>MPFPEKFFWGASSSGFQFEMGDPEGKSIDPNTDWFKWVHDETNIRRGVVSGDLPEHGINYWDLFRSDHELAASIGMNAYRIGIEWSRIFPKPTLDVRVGIELDPEGYITRVEVDDKAIEELDLLANKEAVSRYREIILDLRDRGLKVFVCLNHFTLPLWIHDPIACRDTKLKRGPKGWVDKTTILEFAKYSAYMAWSLGNIVDYWVTFNEPMVVTEAGYFQPEVGFPPGLRNISAFKTACLNIANAHVVAYDLIKKYDKVRADDDSPSAAYVGIVHNIVPIKPYSERKLDLKAADLMNYIHNKWILEFIVRGKIDRSLVGREKYLIDKFKDKLDWLGVNYYTRIVLKGKWVPPLISPVPVIPDIVKGYGFNCTPGGRSLDGMPVSDFGWEVYPQGLSDALDIASEYGKPLIVTENGIADSEDNIRPYFLVSHLKVLEEYVEKKKNVYGYLHWALTDNYEWAQGFKMRFGLTDVDLETKERKPRESSEVFKIIASEKTVPEELVEKYPKPIF[2x]

Beta-glucosidase is an enzyme that catalyzes the hydrolysis of the glycosidic bonds of cellobiose, resulting in the production of glucose, which is an important step for the effective utilization of cellulose. In the present study, a thermostable β-glucosidase was isolated and purified from the Thermoprotei Thermofilum sp. ex4484_79 and subjected to enzymatic and structural characterization. A similarity search was performed with the BLAST program; the TsBGL protein was found to be a member the GH1 family. Members of the GH1 family have a (β/α)8-barrel domain structure that contains the active site, and the hydrolysis of the β-glycosidic bond is carried out via a catalytic mechanism that involves the action of two conserved glutamate residues that act as nucleophiles and proton donors.

The TsBGL crystal belonged to the space group P1211 and diffracted to a resolution of 2.14Å. The asymmetric unit of the crystal structure consisted of two protein molecules. The overall view indicates that TsBGL has a classic (β/α)8-barrel domain structure. The central (β/α)8 barrels consisted of eight parallel β-strands, namely β1 (Phe8-Ser13), β2 (Asn77-Ile83), β3 (Lys146-Asn152), β4 (Asp203-Asn209), β5 (Tyr271-Ile278), β6 (Trp335-Tyr340), β7 (Pro409-Glu414), and β8 (Asn445-His451), surrounded by eight α-helices, namely, α1 (Asn59-Ile74), α2 (Asn126-Arg143), α3 (Lys181-Gly199), α4 (Asn232-Asp258), α5 (Arg287-Asn302), α6 (Pro393-Glu405), α7 (Ile424-Lys444), and α8 (Arg483-Lys496). In TsBGL, Glu210 and Glu414 served as the putative catalytic residues. Glu414 was located at the end of β-strand 7, Glu210 was located behind Asn209, which was the end of β-strand 4, Glu210 is a proton donor, Glu414 is a catalytic nucleophile, and the closest distance between Glu210 and Glu414 was 4.5Å, which matched the catalytic characteristics of GH1 BGLs. The active center of TsBGL was surrounded by aromatic groups and polar residues, including Gln17, His153, Phe154, Asn209, Glu210, Asn339, Tyr341, Glu414, Trp452, Glu459, Trp460, and Phe468. The substitution of either Glu210 or Glu414 with alanine significantly decreased the enzymatic activity. Moreover, TsBGL has approximately 37% of its charged residues involved in ion-pairs, whereas for BGPh, BGTa, and BGSs, 35.2, 41, and 43.2% of its charged residues form ion pairs, respectively. TsBGL exhibited high thermostability, after incubating TsBGL at 85°C for 1.5h, 84% of the activity was retained, and at 90°C, TsBGL retained 47% of its activity for 1.5h.> MALIVQKFGGTSVG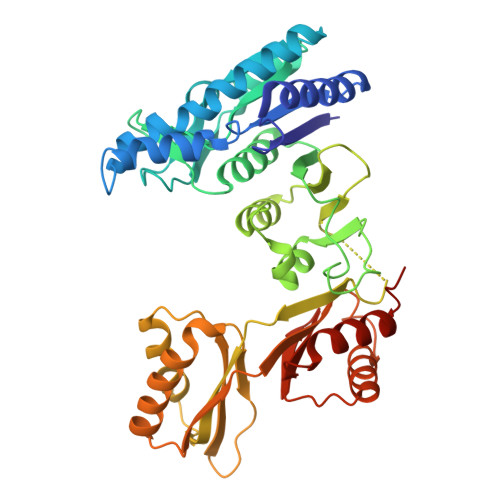TVERIEQVAEKVKKFREAGDDVVVVVSAMSGETNRLIGLANQIMEQPVPRELDVMVSTGEQVTIALLSMALIKRGVPAVSYTGNQVRILTDSAHTKARILHIDDTHIRADLKAGRVVVVAGFQGVDGNGNITTLGRGGSDTTGVALAAALKADECQIYTDVDGVYTTDPRVVPQARRLDKITFEEMLEMASLGSKVLQIRAVEFAGKYNVPLRVLHSFQEGPGTLITIDDEEESMEQPIISGIAFNRDEAKLTIRGVPDTPGVAFKILGPISAANVEVDMIVQNVAHDNTTDFTFTVHRNDYLNALEILKQTAANIGAREAIGDTNIAKVSIVGVGMRSHAGVASRMFEALAKESINIQMISTSEIKVSVVIEEKYLELAVRALHTAFELDAPARQGE>[8x]MGSSHHHHHSSGLVPRGSHMAVIPNFHLPMRSFEVKNRTSVDDIKSLRLITAIKTPYLPDGRFDLEAYDALVNMQIVDGAEGVIVGGTTGEGQLMSWDEHIMLIGHTVNCFGGSIKVIGNTGSNSTREAIHATEQGFAVGMHAALHINP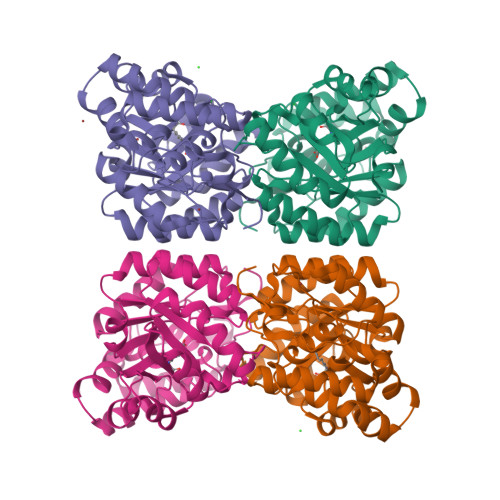YYGKTSLEGLVSHFESVLPMGPTVIYNVPSRTGQDIPPGVIHTVAQSANLAGVKECVGNDRIKQYTDNRIVVWSGNDDQCHDAKWDYGATGVISVTSNLIPGLMRQLLFKGKNPSLNAKIMPLVNWLFEEPNPIGLNTALAQLGVVRPVFRLPYVPLPLAKRVEFVNIVKEIGRENFVGEKDVKVLDDDDFILVGRY> MSLSKVRYGVVSTAKVAPRFIEGVRLAGNGEVVAVSSRTLESAQAFANKYHLPKAYDKLEDMLADESIDVIYVATINQDHYKVAKAALLAGKHVLVEKPFTLTYDQANELFALAESCNLFLMEAQKSVFIPMTQVIKKLLASGEIGEVISISSTTAYPNIDHVTWFRELELGGGTVHFMAPYALSYLQYLFDATITHASGTATFPKGQSDSQSKLLLQLSNGVLVDIFLTTRLNLPHEMIIYGTEGRLIIPHFWKTTHAKLVRNDTSARTIQVDMVSDFEKEAYHVSQMILEGQRVSHIMTPQLTLSGVK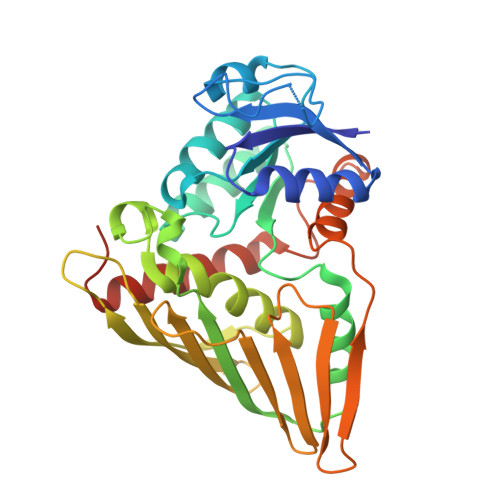IIEDLYRSWGKEGHHHHHH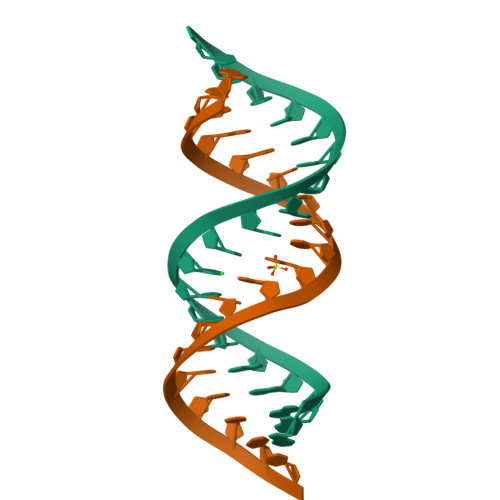>[2x]AGAGAACCCGGAGUUCCCU> TPATGSAEWVIPTVNAKPGEKVTMDVVVKNSAIEVAGAQFNIKQTAPIAYGSAASGDAYAAIVPNETEQYYAFGEGIGK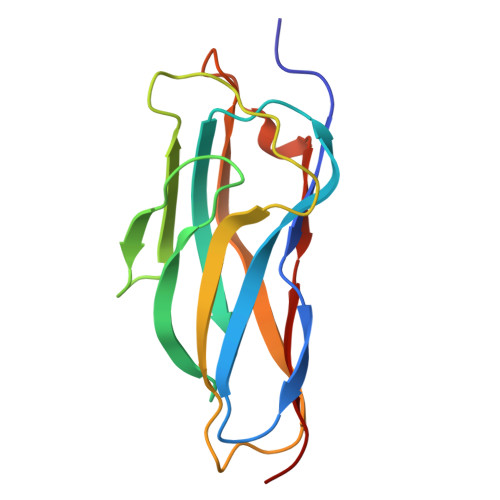GIKAADGAKIITLTFNVPADCAKGTYPVKWSNAFITDTNGNKITDKITLTDGAIVVGDT>GAMNPAAEAEFNILLATDSYKVTHYKQYPPNTSKVYSYFECREKKTENSKLRKVKYEETVFYGLQYILNKYLKGKVVTKEKIQEAKDVYKEHFQDDVFNEKGWNYILEKYDGHLPIEIKAVPEGFVIPRGNVLFTVENTDPECYWLTNWIETILVQSWYPITVATNSREQKKILAKYLLETSGNLDGLEYKLHDFGYRGVSSQETAGIGASAHLVNFKGTDTVAGLALIKKYYGTKDPVPGYSVPAAEHSTITAWGKDHEKDAFEHIVTQFSSVPVSVVSDSYDIYNACEKIWGEDLRHLIVSRSTQAPLIIRPDSGNPLDTVLKVLEILGKKFPVTENSKGYKLLPPYLRVIQGDGVDINTLQEIVEGMKQKMWSIENIAFGSGGGLLQK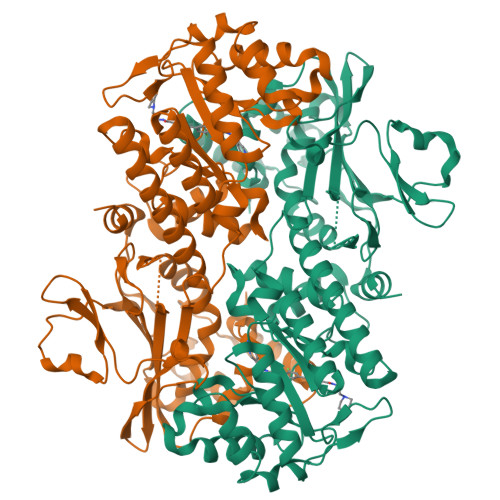LTRDLLNCSFKCSYVVTNGLGINVFKDPVADPNKRSKKGRLSLHRTPAGNFVTLEEGKGDLEEYGQDLLHTVFKNGKVTKSYSFDEIRKNAQLNIELEAAHH[2x]> ATITVSTPIKQIFPDDAFAETIKANLKKKSVTDAVTQNELNSIDQIIANNSDIKSVQGIQYLPNVRYLALGGNKLHDISALKELTNLGWLNLSNNQLETLPQGVFEKLTNLTTLNLSNNQLTSLPQGVFERLASLTTLNLSNNQLTSLPQGVFERLTNLTTLNLSNNQLTSLPQGVFERLTNLTTLNLSNNQLTSLPQGVFERLTSLTTLNLSNNQLTSLPDGVFERLTNLKTLNLSNNQLTKEACRAVANALKQAASLHELHLSNNNIGEEGAAELVEALL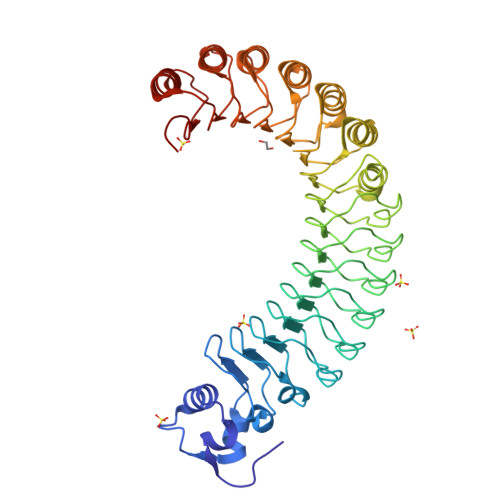HPGSTLETLDLSNCNLTKEACREIARALKQATTLHELHLSNNNIGEEGAAELVEALLHPGSTLETLDLSNCNLTKEACREIARALKQATTLHELHLSNNNIGEEGAAELVEALLHPGSTLETLDLSNCNLTKEACREIARALKQATSLHELHLSNNNIG Peptidyl-prolyl isomerases (PPIases) catalyze intrinsically slow and often rate-limiting isomerization of prolyl-peptide bonds in unfolded or partially folded proteins, thereby speeding up the folding process and preventing misfolding. An example of such a protein is SlyD (Sensitive to Lysis D), which consists of an FKBP type PPIase domain and a chaperone domain, called IF (insert-in-flap) domain, that has been shown to exhibit chaperone activity. Each of these domains contains one binding site for unfolded proteins or peptides. Often, FKBPs are linked to an additional chaperone domain that can increase their PPIase activity by up to 200-fold.

The original S2 peptide sequence (NH2-TRYWNPKMKPFIFGA-COOH) was modified such that the first proline residue was changed to alanine (P6A), a leucine residue was placed upstream of the second proline residue (K9L) and the isoleucine residue was mutated to alanine (I12A), resulting in the pseudo-wild-type (psWT) peptide:NH2-TRYWNAKMLPFAFGA-COOH. Although most of the protein–peptide complexes did not crystallize or yielded crystals of poor diffraction quality, we succeeded in structure determination for four complexes of SlyDWT with bound substrates: psWT, W4A, W4K, and M8A. In all structures, the peptide substrates are bound in the PPIase binding pocket with the proline residue in cis conformation, coordinated by the previously observed protein–peptide polar interactions, namely N35-L9, I37-L9, Y63-F11, H119-F11 and Y92-F13. Although all peptide substrates bound to both SlyDWT domains in solution, the chaperone domains displayed no electron density for peptide substrates psWT and M8A in their respective crystal structures. The absence of these substrates in the high-affinity chaperone domains can be attributed to high dynamics of substrate binding and serendipitous blocking of the binding site by neighbouring molecule of SlyD in the crystal packing. Finally, the residue W4 of psWT peptide could not be resolved, indicating flexibility of the peptide N-terminus. Finally, the loose conformation is defined by the newly determined structures with the substrate bound only in the FKBP domain. In these structures, the access to the FKBP binding site is not restricted and the peptides bound in the FKBP domain can freely diffuse from the binding site upon its release.

> MKVGQDKVVTIRYTLQVEGEVLDQGELSYLHGHRNLIPGLEEALEGREEGEAFQAHVPAEKAYGPHDPEGVQVVPLSAFPEDAEVVPGAQFYAQDMEGNPMPLTVVAVEGEEVTVDFNHPLAGKDLDFQVEVVKVREATPEELLHGHAHPSGHHHHHH;> TRYWNAKMLPFAFGA> MDMTVKKLYFIPAGRCMLDHSSVNSALTPGKLLNLPVWCYLLETEEGPILVDTGMPESAVNNEGLFNGTFVEGQILPKMTEEDRIVNILKRVGYEPDDLLYIISSHLHFDHAGGNGAFTNTPIIVQRTEYEAALHREEYMKECILPHLNYKIIEGDYEVVPGVQLLYTPGHSPGHQSLFIKTEQSGSVLLTIDASYTKENFEDEVPFAGFDPELALSSIKRLKEVVKKEKPIIFFGHDIEQEKSCRVF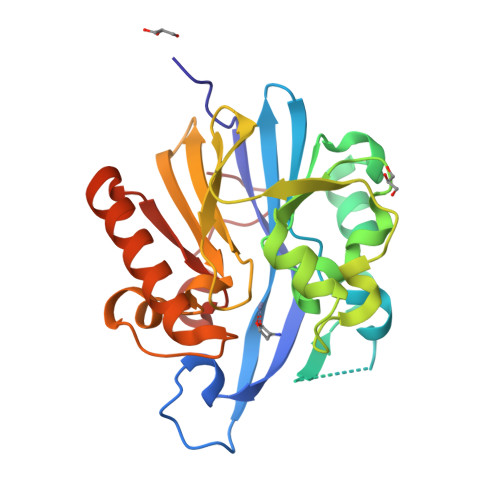PEYI>MGWSDHDELSTDTTLHEEKFRIEPVPVHHQLDILKIAVSENYKTFASVGLDRCLVVWDLRQWCTKLVLSKEQMPRTLKAIALDPQGNYVSLFSKDTLFILNVESPSLMLQHSYHCKPNSKLNVFWMPGTHKDDEWKNFELVVVESSGEIQVFSLTIEIEGADIALVEKFQLSSPIIKSISIVSPTANRIACLTESGEVTVYSKKGPVWSPKILSQNKNYLTETKKDIYGIAMADILFLARDSGVDMIDLKNDELLHSFTLPPIKVNTFSVGVSNSRFVNGQFRVSSISFCFTHAVTEKVLYYYYGNESNESYIILNKWDQQPNLVDVHDPDNSLASLTFDELQENIHEVEDASESVMSSDGLYIFGMRRKSSSGISPTADEKNEDNGFTLRNRKLR[4x];>[4x]AHMQHSKSSVHAELRELPESTANLIENSHADDVFSPNMVERLWVLAKSTRDSAQMSDSIISSLSDVLVL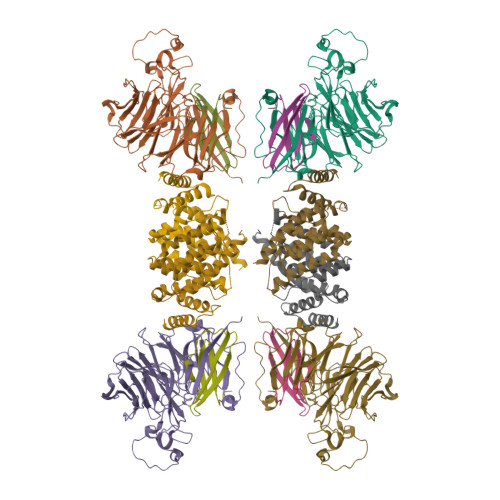SPLEVLASWYAADLLDALLMESLSRKVEISEIEEIISLCPKNSSIIRHALLAKLVLFPENTADSLNEVLAAYKNTLDLCSQDKRKQSSVLKINLSKLFTLHSCLSLALQRLGYGDVSKRMYQEIFVPDSDADITPLSFIISWTALNTFAPICTSPKENDVVEKMAMYVRTAIGTLKIQDLKLSRKLINSCIDIGSRLQEDLGY;>AHMNTHSGGETQVWEVWMYSQSEKKHRSKSLKMYNSLIIADPGPSLAVSDRCVAIVLGNYVALVGYGSEIFRDFYQIRNSDEMDRILRRKRKNLQRKRSGTIG[4x]>MGLAVFLPPYPFRGLKAPYLWMFYKYLHCATDSILFITGEDYLSVTDDEAQRARWEFDPASMASLGYELPNAQSMACHEYLTLDNAFYETLLSRHHHDPIKSFSAFLTERIPDLETELHALLDSKKGIIDQIDTFISICNCPSLEHVARTLGKEVMHIEIGPLRAPMYRNTAYLDFAGVNGGTEASARYEKCQAEFDIKASLGDLHNYFLEVLPPAEAATHSAAGVVLQVEDCSNLIAYNHDFTNISLLSYVRQRYEKEDI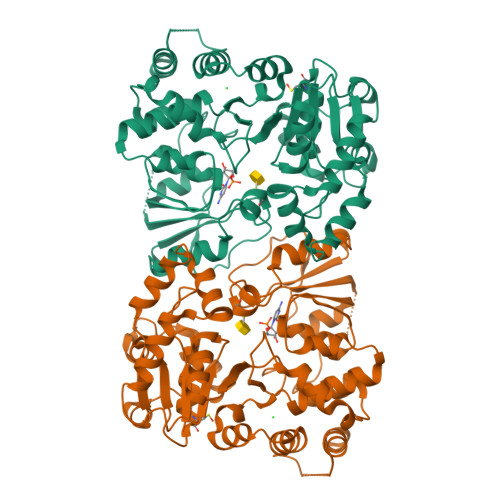LVRAHPGSLFRLRDDVFTIDDSANSLAFINQCNEVFTINSSVGLEAILTGKKTTVLGDCSYAFINELAGASATVNAAAFYLFSYLVPFDLVFNQEYLKFRLGHPEEREIVGKHIEFYSADMPGSLSQAAHSLSSLINEAISLEHHHHHH[2x]>GGCACUGG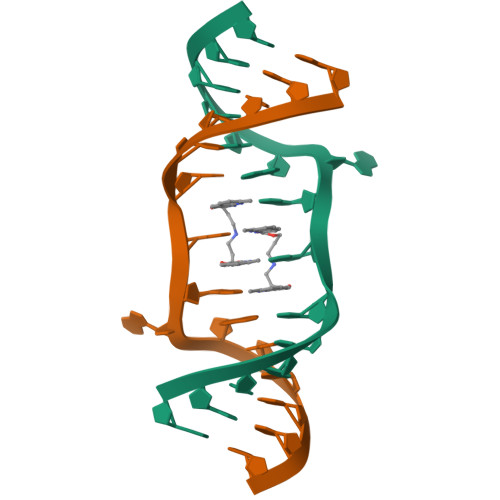AAGUGCC[2x]2-[(1E,3E,5E,7E,9E,11E,13E,15E,17E,19E)-3,7,12,16,20,24-hexamethylpentacosa-1,3,5,7,9,11,13,15,17,19,23-undecaenyl]-1,3,4-trimethyl-benzene | C40 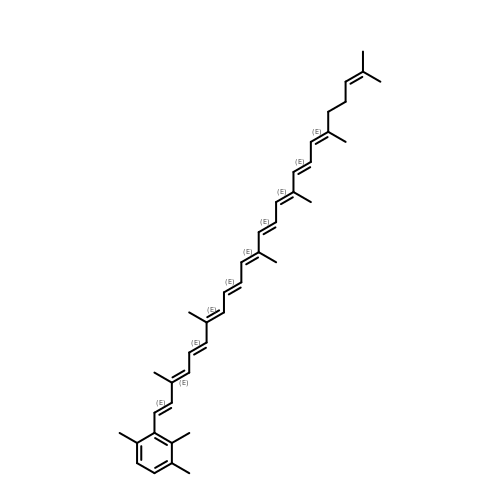H52 | VJASLAGEYVTOGS-IQAIWTHGSA-N>[3x]MKKLVKLAAFGAAAAVAATLGAIAPASAHGEKSQQAFLRMRTLNWYDVQWSKTTVNVNEEMILSGKVHVFSAWPQAVANPRVSFLNAGEPGPVLVRTAQFIGEQFAPRSVSLEIGKDYAFSINLRGRRAGRWHVHAQINVEGGGPIIGPGQWIEIKGDMKDFTDPVTLLDGSTVDLENYGISRIYAWHLPWLAVGAAWILFWFIRKGIIASYVRVAEGRPDDVIGDDDRRIGAIVLALTILATIVGYAVTNSTFPRTIPLQAGLQKPLTPIETEGTVGVGKEQVTTELNGGVYKVPGRELTINVKVKNGTSQPVRLGEYTAAGLRFLNPTVFTQKPDFPDYLLADRGLSNDDVIAPGESKEIVVKIQDARWD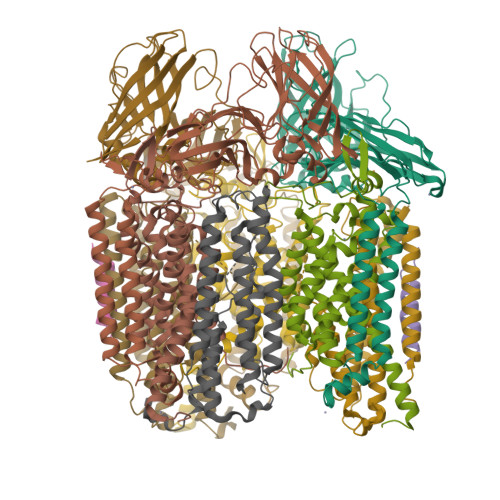IERLSDLAYDTDSQVGGLLFFFTPDGKRFAAEIGGPVIPKFVAGDMP;>MSQSKSGGAVGPFNSVAEAAGCVATTDWMLLVLLFFAVLGGYHVHFMLTAGDWDFWVDWKDRRMWPTVLPILGVTFCAASQAFWWVNFRLPFGAVFAVLGLMIGEWINRYVNFWGWTYFPISLVFPSAMIVPAIWLDVILLLSGSYVITAVVGSLGWGLLFYPNNWPAIAAFHQATEQHGQLMTLADLIGLHFVRTSMPEYIRMVERGTLRTFGKDVVPVAAFFSGFVSMMVYFLWWFMGRWYSTTKRIEQI[3x];>[3x]MSSTTSTAAGAAAEVESVVDLRGMWIGLAVLNVFYLIVRIYEQVFGWRAGLDSFAPEFQTYWMSILWTEIPLELVSGLGLAGYLWKTRDRNVDAVAPREEMRRLVVLVQWLVVYGIAIYWGASFFTEQDGAWHMTVIRDTDFTPSHIIEFYMSYPIYSVIAVGAFFYAKTRIPYFAHGYSLAFLIVAIGPFMIIPNVGLNEWGHTFWFMEELFVAPLHWGFVFFGWMALGVFGVVLQILGRIHALIGKEGVALLTE;>AAAAAAAAAAAAAAAAAAA[2x]>[2x]MSYYHHHHHHLESTSLYKKAGLENLYFQGVKIMPNLPGLYFLQAYPSEEIWRLFVDGRFWSKENGWRGYESREPGCLNAALESLCSIALQVEKSGEEFELSVDLIKRIHKKCGKKVEELQEKNPGELRTDEPVSFGIPAGRASIKGIEEFLSLVFLTEGGAEFGPGKAGPFGPRFDKNYFKNLNPEQIPDLAKQIYFDMCKYGHSNTNHFYLAVMKNVDVYLEKITQSYNKEIKTAETLDEKLKIIVKHIRMYEVLHPFRDANGRTFVNNLLNIPLMQQGLPPATFYEPNVFDLYSAEELVVVVKEAIFNTVEIIEQSKRKTPITLYGYHSSLEEQTKFRDMLDSPSYEKIKHMDFSDLNPEKLHLKTQKCLSSLNEQYPLHRGAIYLSDPGEIKLLLSNRNESQINQQIEQGAPPIYVGKTPAHLAVISGNMAMLDELIAKKADLSLQDYDGKTALHYAAECGNMQI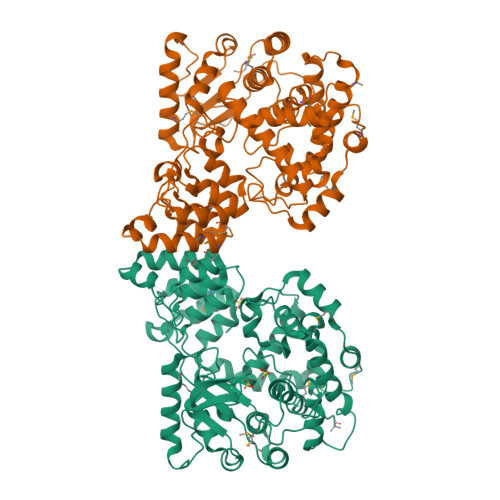MGKILKVVLSQEDAIKVLNIKDNHGKTAFHYAAEFGTPELISAL In these environments, biology utilizes a finely tuned protein catalyst termed the mercuric reductase (MerA) (encoded by the merA gene) in order to reduce toxic ionic mercury (Hg2+) to the far less toxic, volatile, and elemental form (Hg0). The reaction catalyzed by MerA follows the reaction scheme of NADPH + Hg2+ → NADP+ + Hg0. Structural characterization confirmed that MerA is a member of the DSOR protein family, which adopts a βαββαβ fold, and which is known to catalyze pyridine-dependent substrate reduction with a characteristic active site CXXXXC motif. Here, we report biochemical and structural characterization of a thermostable MerA from the aerobic thermoacidophilic Crenarchaeon Mse (MseMerA).

The crystal structure of MseMerA was solved to 1.6 Å, with R and Rfree values of 16.9 and 19.6%, respectively. Bound FAD was observed, suggesting that these molecules act to stabilize the structure. No mercury was observed in the active site. As expected based on the sequence alignment, a clear reduction in loop regions was observed in comparison to Tn501MerA. No electron density for the carboxy terminus of MseMerA was identified from 440 to 448, including the conserved pair of cysteines at residues 446 and 447. This is in agreement with the carboxy terminus being able to undergo conformational changes during the catalytic cycle. The structure of MseMerA reveals a dimeric biological assembly, as has been shown with previous structures. With this architecture, the active site cleft on one monomer interacts with the C-terminal domain of the opposing monomer. In contrast, in MseMerA, the F441′ in the position of tyrosine in Tn501MerA lacks a hydroxyl group to coordinate the Hg2+ ion, but a glutamic acid in place of the Tn501MerA V317 provides a different residue with which the Hg2+ ion could potentially be coordinated. Retention of 100% activity after incubation at 97°C for 100 min further confirms the highly thermostable nature of MseMerA.

> MGSSHHHHHHSQDPMHKLAIIGYGAAGFAAMIKANELGVKPVLIGKGEIGGTCVNVGCVPSKRMLYIAEIYKKAREVTGSEVYPPFSSFQEKDGLVQEMRKTKYEDLLSYYDVELIQGEARFISPHAVKVNGQVIEAEKFVIATGSSPLIPRIPGLDKVGFWTNREALSPDRRIDSLAVIGGRALALEFAQMYSRMKVEVAILQRSPVLIPDWEPEASVEARRIMENDGVAVVTGVNVKEVRKGAGKIVITDKGEVEADEILLATGRKPNVDLGLENAGVRLNERGGIKVDDELRTDNPHIYAAGDVLGGKMLEALAGRQGSIATENALTGSHKRVDENAVPQVIFTQPNLARVGLTEAEARAKEGEVEARVLPMSSVAKAEIINSRLGFVKMVTMNGRIVGVHAVGENVAEMIGEAALAIRFGATVHDLIDTVHMFPTIAESLRLVALAFRSDVSRLSCCV URACIL-6-ACETIC ACID | C6 H6 N2 O4 | 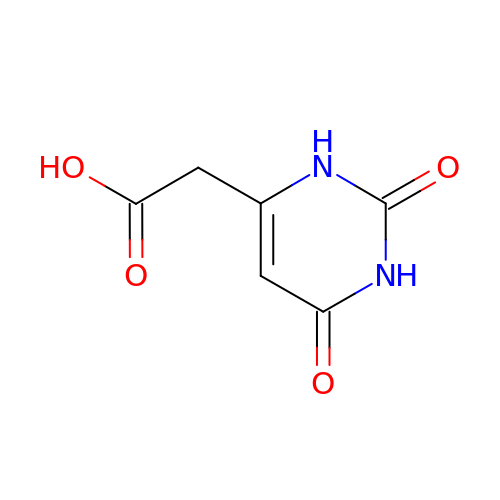NQAUNZZEYKWTHM-UHFFFAOYSA-N>MRPALYFCGSIRGGREDRTLYERIVSRLRRFGTVLTEHVAAAELGARGEEAAGGDRLIHEQDLEWLQQADVVVAEVTQPSLGVGYELGRAVAFNKRILCLFRPQSGRVLSAMIRGAADGSRFQVWDYEEGEVEAL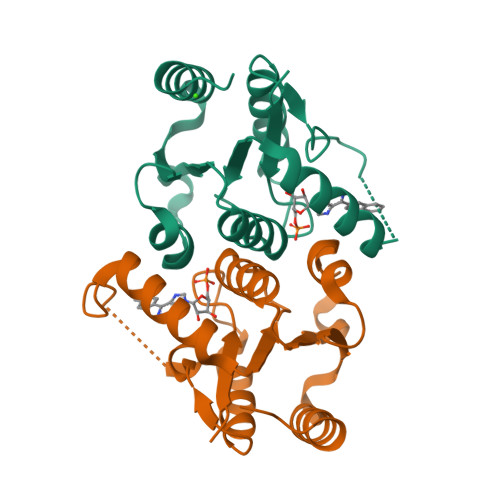LDRYFEADPLEHHHHHH[2x]2-(1H-1,2,3-triazol-1-yl)ethyl 6-deoxy-alpha-L-galactopyranoside | 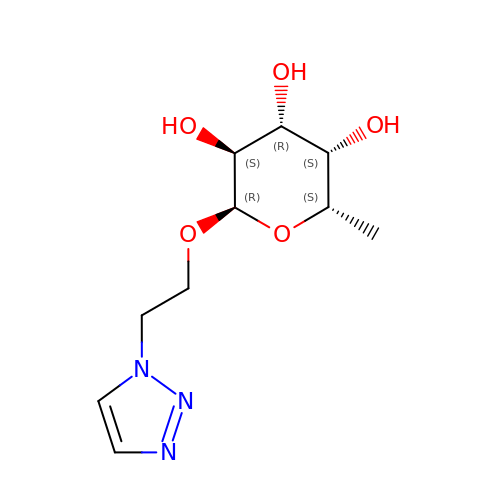C10 H17 N3 O5 | AQLGVIQGWAYMPY-LOLPMWEVSA-N>[2x]GLTAAQIKAIQDHWFLNIKGCLQAAADSIFFKYLTAYPGDLAFFHKFSSVPLYGLRSNPAYKAQTLTVINYLDKVVDALGGNAGALMKAKVPSHDAMGITPKHFGQLLKLVGGVFQEEFSA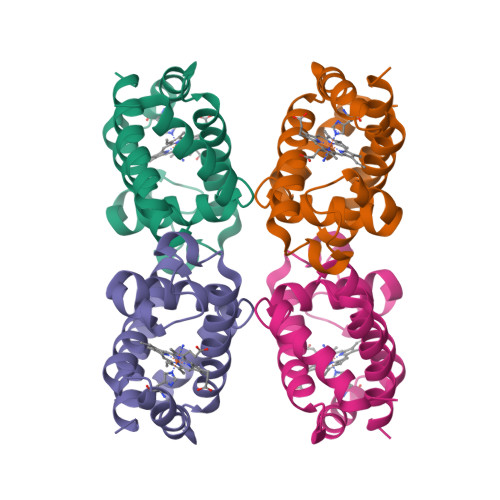DPTTVAAWGDAAGVLVAAMK>MAHHHHHHHHHHGALEVLFQGPGDPTVFHKRYLKKIRDLGEGHFGKVSLYCYDPTNDGTGEMVAVKALKADAGPQHRSGWKQEIDILRTLYHEHIIKYKGCCEDAGAASLQLVMEYVPLGSLRDYLPRHSIGLAQLLLFAQQICEGMAYLHSQHYIHRDLAARNVLLDNDRLVKIGDFGLAKAVPEGHEYYRVREDGDSPVFWYAPECLKEYKFYYASDVWSFGVTLYELLTHCDSSQSPPTKFLELIGIAQGQMTVLRLTELLERGERLPRPDKCPAEVY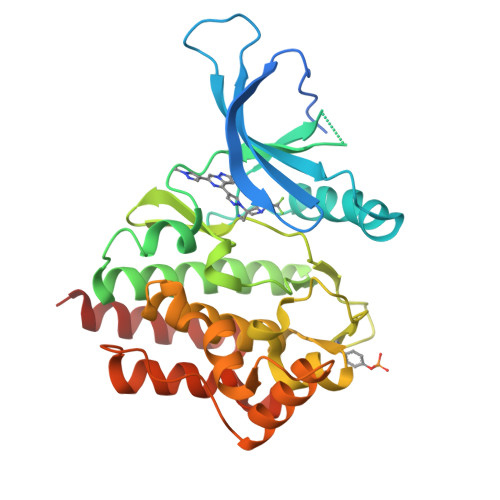HLMKNCWETEASFRPTFENLIPILKTVHEKYQGQAPS[2x]> MIYMTFGEILKKERVSWKLSVKELSTLSGVSQTYISKLENGKRNFPSLETIFNLLIGFKTHIEYKMGSESPFYEINNSYLDEILIMFINSSNSTISDRDPNELITQFNEYYDVTIKKKQNENSKIESDIFSNKIKLVKGTTKKEVIEKPYFDLNWLLTQNEYEVFFDRSFLLDNNFLNKKHFTEKDMYYYNVLNDNDLKTIKDEIVVFLLNKYNYIKNKDDFFNIFTNSEDDKTKRDALYKILYETD;> GAMDPMVTKEFLKIKLECSDMYAQKLIDEAQGDENKLYDLFI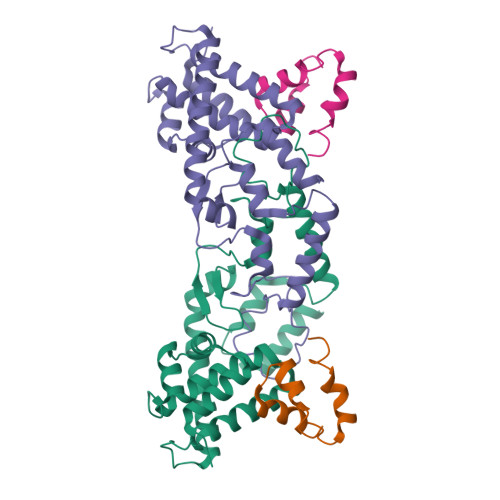QKLAERHTRPAIVEY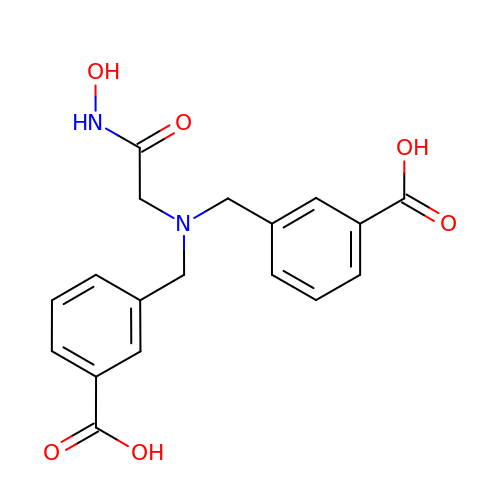3-[[(3-Carboxyphenyl)methyl-[2-(hydroxyamino)-2-oxoethyl]amino]methyl]benzoic acid | C18 H18 N2 O6 | KHSBLMDTVROJFV-UHFFFAOYSA-N> ARAKVTMNDFDYLKLLGKGTFGKVILVREKATGRYYAMKILRKEVIIAKDEVAHTVTESRVLQNTRHPFLTALKYAFQTHDRLCFVMEYANGGELFFHLSRERVFTEERARFYGAEIVSALEYLHSRDVVYRDI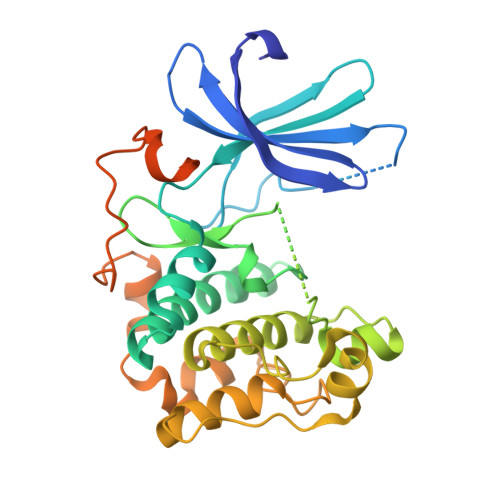KLENLMLDKDGHIKITDFGLCKEGISDGATMKTFCGTPEYLAPEVLEDNDYGRAVDWWGLGVVMYEMMCGRLPFYNQDHERLFELILMEEIRFPRTLSPEAKSLLAGLLKKDPKQRLGGGPSDAKEVMEHRFFLSINWQDVVQKKLLPPFKPQVTSEVDTRYFDDEFTAQSITITPPDRYDSLGLLELDQRTHFPQFSYSASIRE> MISDSMTVEEIRLHLGLALKEKDFVVDKTGVKTIEIIGASFVADEPFIFGALNDEYIQRELEWYKSKSLFVKDIPGETPKIWQQVASSKGEINSNYGWAIWSEDNYAQYDMCLAELGQNPDSRRGIMIYTRPSMQFDYNKDGMSDFMCTNTVQYLIRDKKINAVVNM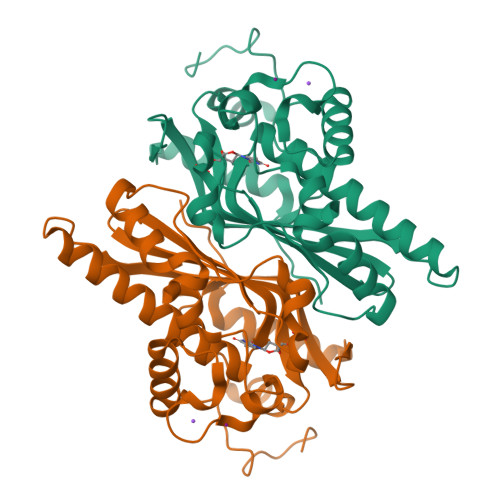RSNDVVFGFRNNYAWQKYVLDKLVSDLNAGDSTRQYKAGSIIWNVGSLHVYSRHFYLVDHWWKTGETHISKKDYVGKYALEHHHHHHHH TRPV3 is most abundantly expressed in epidermal and hair follicle keratinocytes where it plays a key role in the maintenance of normal skin physiology. In contrast to other thermoTRP channels, TRPV3 sensitizes, rather than desensitizes, upon repeated stimulation with either heat or agonists. The TRPV3 channel, like other thermoTRPV channels (TRPV1, TRPV2, and TRPV427–30), is a fourfold symmetric homotetramer. Each monomer contains an amino- (N-) terminal cytosolic ankyrin repeat domain (ARD) and a domain-swapped transmembrane domain (TMD) comprising six transmembrane helices (S1−S6).

To elucidate the conformational changes governing transition of TRPV3 from the closed to the open state, we determined structures of the channel in the presence of the agonist 2-APB (TRPV32-APB). A single cryo-EM dataset yielded three distinct conformations, TRPV32-APB 1, TRPV32-APB 2, and TRPV32-APB 3, all of which resolved to ~4 Å resolution or better. Strikingly, two out of the three TRPV32-APB structures exhibit twofold (C2) symmetry (TRPV32-APB 2, and TRPV32-APB 3), deviating from the canonical fourfold (C4) symmetry previously associated with thermoTRPV channels. The reduced symmetry is conspicuous in the pores of the TRPV32-APB 2 and TRPV32-APB 3 structures, where movement in the C-terminal region of S6 in diagonally opposing protomers results in asymmetric gate arrangements within the channels. In TRPV32-APB 2 the distance between the M677 residues in subunits A and C is ~5.7 Å, similar to the diameter of the closed gate of apo TRPV3 (~5.2 Å). However, in subunits B and D this distance is increased to ~9.1 Å which is similar to the ~9.3 Å diameter measured between gate residues in the structure of TRPV1 bound to double-knot toxin (DkTx) and resiniferatoxin (RTx). However, TRPV32-APB 2 is likely to be nonconductive, as the narrow opening of subunits A and C constricts the pore. It is thus possible that this arrangement of subunits represents an intermediate state. Interestingly, an overlay of S5 helices of subunits A and B revealed that their S4−S5 linkers contain π-helices that originate at two different positions: at residue I583 in subunit A and at residue M578 in subunit B. Since the π-helices dictate the angle between subunits, it is likely that the differing positions of S4−S5 π-helices within the tetramer are responsible for the twofold symmetric arrangement of the channel.

>[4x]MEKAHPKEMVPLMGKRVAAPSGNPAILPEKRPAEITPTKKSAHFFLEIEGFEPNPTVAKTSPPVFSKPMDSNIRQCISGNCDDMDSPQSPQDDVTETPSNPNSPSAQLAKEEQRRKKRRLKKRIFAAVSEGCVEELVELLVELQELCRRRHDEDVPDFLMHKLTASDTGKTCLMKALLNINPNTKEIVRILLAFAEENDILGRFINAEYTEEAYEGQTALNIAIERRQGDIAALLIAAGADVNAHAKGAFFNPKYQHEGFYFGETPLALAACTNQPEIVQLLMEHEQTDITSRDSRGNNILHALVTVAEDFKTQNDFVKRMYDMILLRSGNWELETTRNNDGLTPLQLAAKMGKAEILKYILSREIKEKRLRSLSRKFTDWAYGPVSSSLYDLTNVDTTTDNSVLEITVYNTNIDNRHEMLTLEPLHTLLHMKWKKFAKHMFFLSFCFYFFYNITLTLVSYYRPREEEAIPHPLALTHKMGWLQLLGRMFVLIWAMCISVKEGIAIFLLRPSDLQSILSDAWFHFVFFIQAVLVILSVFLYLFAYKEYLACLVLAMALGWANMLYYTRGFQSMGMYSVMIQKVILHDVLKFLFVYIVFLLGFGVALASLIEKCPKDNKDCSSYGSFSDAVLELFKLTIGLGDLNIQQNSKYPILFLFLLITYVILTFVLLLNMLIALMGETVENVSKESERIWRLQRARTILEFEKMLPEWLRSRFRMGELCKVAEDDFRLCLRINEVKWTEWKTHVSFLNEDPGPVRRTDFNKIQDSSRNNSKTTLNAFEEVEEFPETSVVDAGLEVLFQGPAAAVDYKDDDDKAHHHHHHHHHH> MHHHHHHLEVLFQGPSGMSVDQATLDKLEAGFKKLQDAKDCKSLLKKYLTKEIFDRLKTRKTAMGATLLDVIQSGVENLDSGV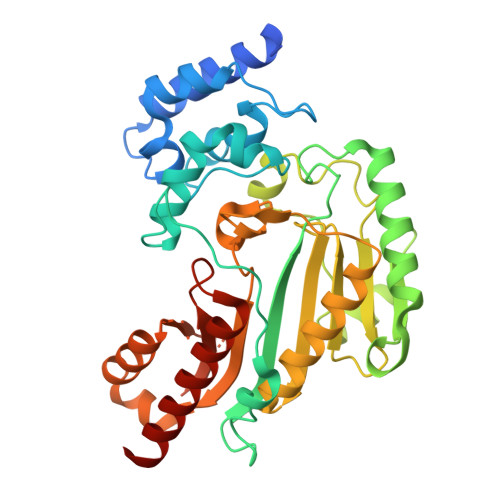GVYAPDAESYTVFADLFDPVIEDYHGGFKPTDKHPPTDFGDMNTIVNVDPENKYVVSTRVRCGRSLQGYPFNPCLTEAQYKEMEDKVSSQLKGMTGDLKGTYYPLTGMDKKTQQQLIDDHFLFKEGDRFLQAANACRYWPTGRGIYHNDAKTFLVWVNEEDHLRIISMQQGGDLKQVYSRMVSGVKEIEKKLPFSRDDRLGFLTFCPTNLGTTIRASVHIKLPKLAADKAKLDSIAAKYNLQVRGTRGEHTESEGAVYDISNKRRMGLTEYQAVREMQDGIQELIKLEQAA>[4x]MATIVNLLVGGPTANYPADLTTIPGPWVGADRGALR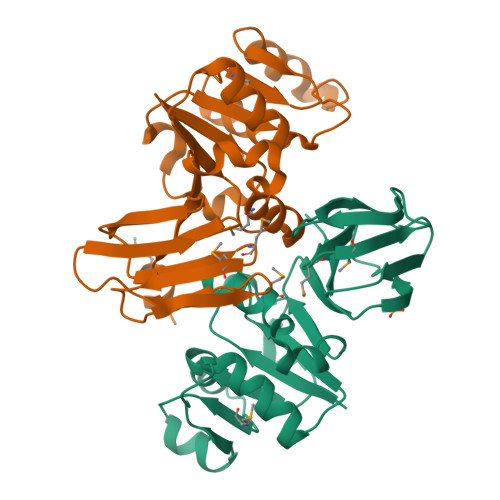LVKRGIQPVMVVGDFDSIDAAELQTVKDALVGAIVVKPDQDHTDTQLAIKSIFEQLQPDEVHLYGATGGRLDHLLANMWLVLDPVFRQWAPQIKLIDKQNSVRFFLPGDYQITKEADKRYLAFVPLMPMHLTLPDEKYQLDAAYNAYPISWASNEFSGNTGHFSFDAGVLAVIQSRDDSMADALEHHHHHH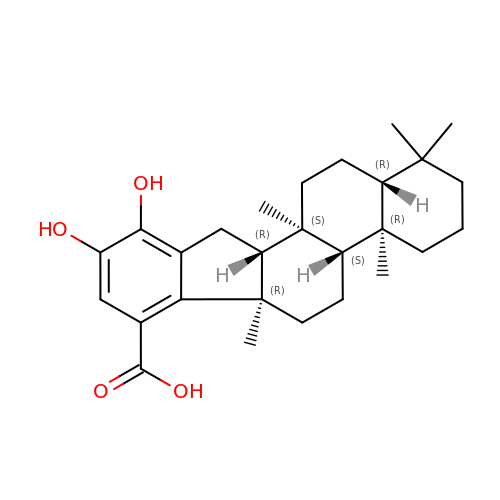(4~{a}~{R},4~{b}~{S},6~{a}~{R},11~{a}~{R},11~{b}~{S},13~{a}~{R})-1,1,4~{a},6~{a},11~{b}-pentamethyl-9,10-bis(oxidanyl)-3,4,4~{b},5,6,11,11~{a},12,13,13~{a}-decahydro-2~{H}-indeno[2,1-a]phenanthrene-7-carboxylic acid | C27 H38 O4 | VSODJBVPHOOTEU-OBYLJCASSA-N>QEASLFLVGERLNATGSKRFREMLFARDLEGILALAREQVEEGAHALDLSVAWTGRDELEDLRWLLPHLATALTVPVMVDSTSPEAMELALKYLPGRVLLNSANLEDGLERFDRVASLAKAHGAALVVLAIDEKGMAKTREEKVRVALRMYERLTEHHGLRPEDLLFDLLTFPITQGDEESRPLAKETLLAMEELRERLPGVGFVLGVSNVSFGLKPRARRVLNSVFLDEARKRGLTAAIVDAGKILPISQIPEEAYALALDLIYDRRKEGFDPLLAFMAYFEAHKEDPGKREDAFLALPLLERLKRRVVEGRKQGLEADLEEALKAGHKPLDLINGPLLAGMKEVGDLFGAGKMQLPFVLQAAEVMKRAVAYLEPHMEKKGEGKGTLVLATVKGAVHDIGKNLVDIILSNNGYRVVNLGIKVPIEEILKAVEAHKPHAVGMSGLLVKSTLVMKENLEYMRDRGYTLPVILGGAALTRSYVEELRAIYPNVYYAEDAF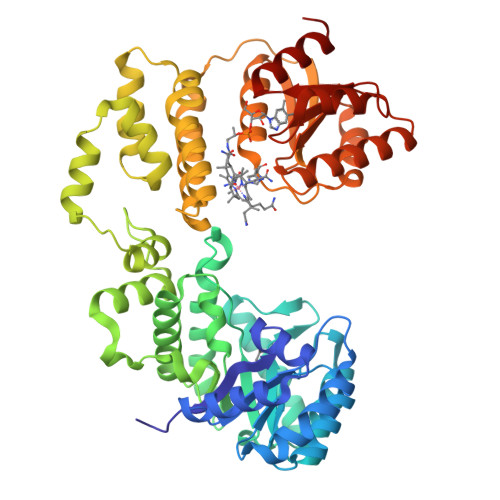EGLRLMEELTGHA[6x]>DVSGTVCLSALPPEATDTLNLIA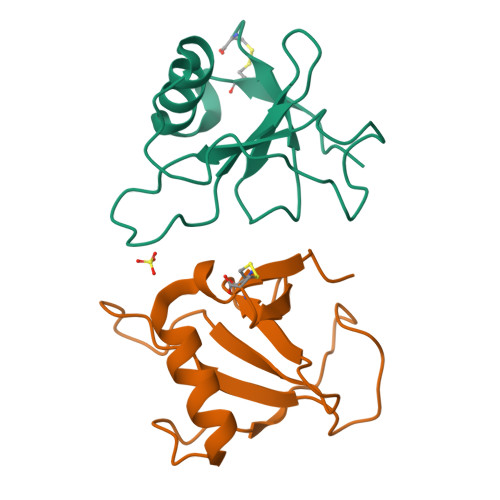ADGPFPYSQDGVVFQNRESVLPTQSYGYYHEYTVITPGARTRGTRRIITGEATQEDYYTGDHYATFSLIDQTC[2x]> MGSDKIHHHHHHMEADRGRNNKVRCAVVDTNVLMYVYLNKADVVGQLREFGFSRFLITASVKRELEKLEMSLRGKEKVAARFA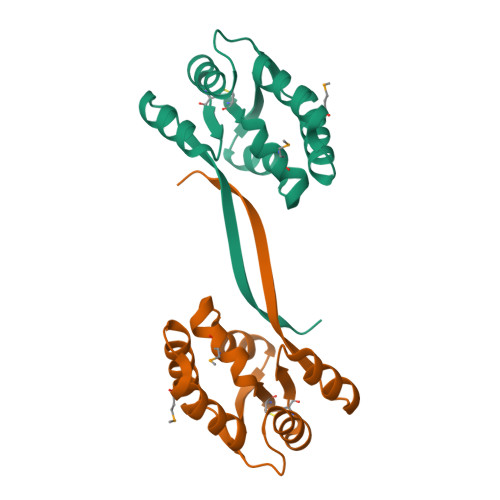LKLLEHFEVVETESEGDPSLIEAAEKYGCILITNDKELKRKAKQRGIPVGYLKEDKRVFVELLD2'-deoxy-5'-O-[(R)-hydroxy{[(R)-hydroxy(phosphonooxy)phosphoryl]methyl}phosphoryl]uridine | C10 H17 N2 O13 P3 | 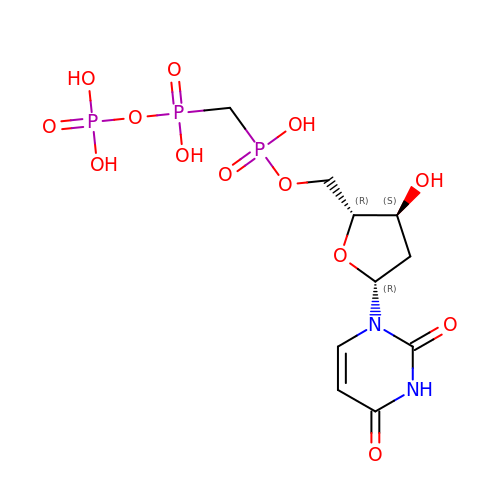CLYYXAGDTAZMBH-LKEWCRSYSA-N>[4x]GPRARDLGVPFEGTPGALNAITDVAGVEVGHTTVISGDGAMVIGKGPYRTGVTIIHPLGKTS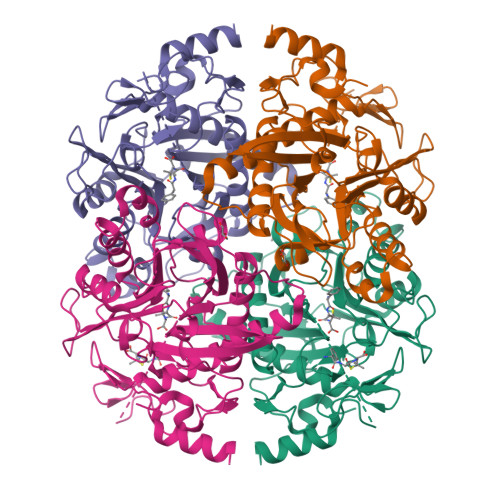LDGVAAGRAVINGTGEWTGMHLVDEVGQFLGPIALTGTGNVGLVHQSMMDWSVGKVPEEALFSRLLPVVAETLDNRLNDVFGHGLTRDHVFAALDGAKGGPVAEGNVGGGTGMIAYTFKGGIGTSSRVVSAGDTRYTVGVLVQANHGDRNDLRIAGVQIGKEIKGAWPEVNGIVAAGPDAGKPQDKNSLLIVIATDAPLMPHQLERMARRAALGVGRNGSTAGALSGEFALAFSTSHVIPLGGKPRLPAIINDTDSETMNALFRGVVQATEEALVNQLVASETMTGANNAKVYGIPHDQLARIMKARFPRR>IIEEEQQSLTGRLNIAVLPTIAPYLLPRVFPIWKKELAGLEIHVSEMQTSRCLASLLSGEIDMAIIASKAETEGLEDDLLYYEEFLGYVSRCEPLFEQDVIRTTEVNPHRLWLLDEGHCFRDQLVRFCQMKGLHERQ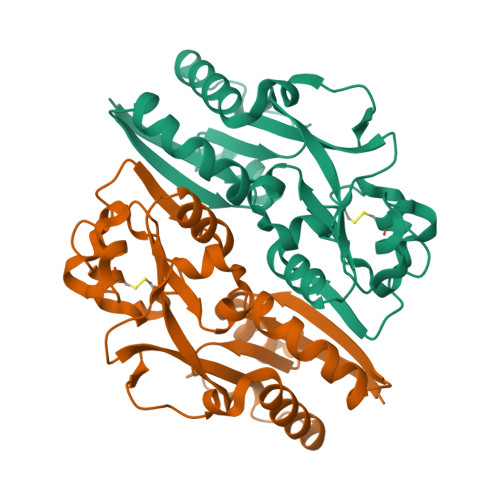TAYSGGSMEAFMRLVESGQGITFIPQLTVEQLSPSQKELVRPFGMPRPVREVRLAVRQDYSRRKLREQLIGLLRSAVPSDMHKLQTGQHLAHHHH[2x]2-{(Z)-[(2-hydroxynaphthalen-1-yl)methylidene]amino}-N-[(1S)-1-phenylethyl]benzamide 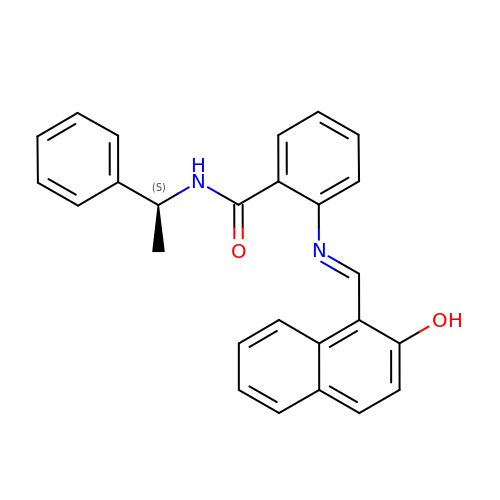| C26 H22 N2 O2 | UXJFDYIHRJGPFS-PTXYPZRJSA-N>[2x]MISHSELRKLFYSADAVCFDVDSTVIREEGIDELAKICGVEDAVSEMTRRAMGGAVPFKAALTERLALIQPSREQVQRLIAEQPPHLTPGIRELVSRLQERNVQ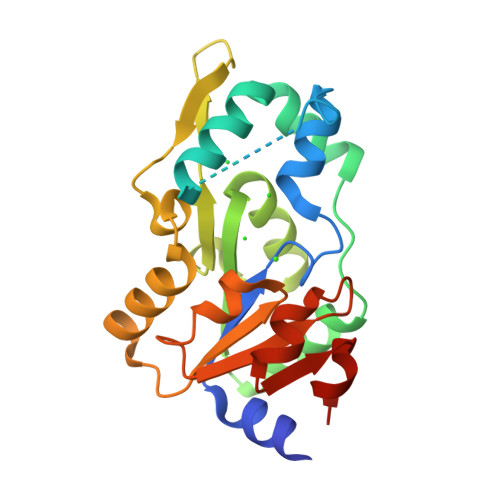VFLISGGFRSIVEHVASKLNIPATNVFANRLKFYFNGEYAGFDETQPTAESGGKGKVIKLLKEKFHFKKIIMIGDGATDMEACPPADAFIGFGGNVIRQQVKDNAKWYITDFVELLGELEE> MTIHEHDRVSADRGGDSPHTTHALVDRLMAGEPYAVAFGGQGSAWLETLEELVSATGIETELATLVGEAELLLDPVTDELIVVRPIGFEPLQWVRALAAEDPVPSDKHLTSAAVSVPGVLLTQIAATRALARQGMDLVATPPVAMAGHSQGVLAVEALKAGGARDVELFALAQLIGAAGTLVARRRGISVLGDRPPMVSVTNADPERIGRLLDEFAQDVRTVLPPVLSIRNGRRAVVITGTPEQLSRFELYCRQISEKEEADRKNKVRGGDVFSPVFEPVQVEVGFHTPRLSDGIDIVAGWAEKAGLDVALARELADAILIRKVDWVDEITRVHAAGARWILDLGPGDILTRLTAPVIRGLGIGIVPAATRGGQRNLFTVGATPEVARAWSSYAPTVVRLPDGRVKLSTKFTRLTGRSPILLAGMTPTTVDAKIVAAAANAGHWAELAGGGQVTEEIFGNRIEQMAGLLEPGRTYQFNALFLDPYLWKLQVGGKRLVQKARQSGAAIDGVVISAGIPDLDEAVELIDELGDIGISHVVFKPGTIEQIRSVIRIATEVPTKPVIMHVEGGRAGGHHSWEDLDDLLLATYSELRSRANITVCVGGGIGTPRRAAEYLSGRWAQAYGFPLMPIDGILVGTAAMATKESTTSPSVKRMLVDTQGTDQWISAGKAQGGMASSRSQLGADIHEIDNSASRCGRLLDEVAGDAEAVAERRDEIIAAMAKTAKPYFGDVADMTYLQWLRRYVELAIGEGNSTADTASVGSPWLADTWRDRFEQMLQRAEARLHPQDFGPIQTLFTDAGLLDNPQQAIAALLARYPDAETVQLHPADVPFFVTLCKTLGKPVNFVPVIDQDVRRWWRSDSLWQAHDARYDADAVCIIPGTASVAGITRMDEPVGELLDRF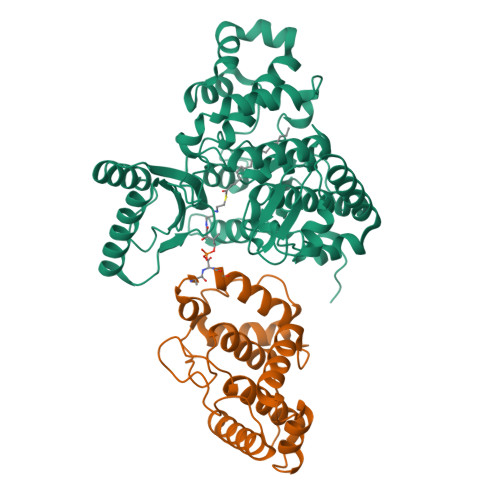EQAAIDEVLGAGVEPKDVASRRLGRADVAGPLAVVLDAPDVRWAGRTVTNPVHRIADPAEWQVHDGPENPRATHSSTGARLQTHGDDVALSVPVSGTWVDIRFTLPANTVDGGTPVIATEDATSAMRTVLAIAAGVDSPEFLPAVANGTATLTVDWHPERVADHTGVTATFGEPLAPSLTNVPDALVGPCWPAVFAAIGSAVTDTGEPVVEGLLSLVHLDHAARVVGQLPTVPAQLTVTATAANATDTDMGRVVPVSVVVTGADGAVIATLEERFAILGRTGSAELADPARAGGAVSANATDTPRRRRRDVTITAPVDMRPFAVVSGDHNPIHTDRAAALLAGLESPIVHGMWLSAAAQHAVTATDGQARPPARLVGWTARFLGMVRPGDEVDFRVERVGIDQGAEIVDVAARVGSDLVMSASARLAAPKTVYAFPGQGIQHKGMGMEVRARSKAARKVWDTADKFTRDTLGFSVLHVVRDNPTSIIASGVHYHHPDGVLYLTQFTQVAMATVAAAQVAEMREQGAFVEGAIACGHSVGEYTALACVTGIYQLEALLEMVFHRGSKMHDIVPRDELGRSNYRLAAIRPSQIDLDDADVPAFVAGIAESTGEFLEIVNFNLRGSQYAIAGTVRGLEALEAEVERRRELTGGRRSFILVPGIDVPFHSRVLRVGVAEFRRSLDRVMPRDADPDLIIGRYIPNLVPRLFTLDRDFIQEIRDLVPAEPLDEILADYDTWLRERPREMARTVFIELLAWQFASPVRWIETQDLLFIEEAAGGLGVERFVEIGVKSSPTVAGLATNTLKLPEYAHSTVEVLNAERDAAVLFATDTDPEPEPEEDEPVAESPAPDVVSEAAPVAPAASSAGPRPDDLVFDAADATLALIALSAKMRIDQIEELDSIESITDGASSRRNQLLVDLGSELNLGAIDGAAESDLAGLRSQVTKLARTYKPYGPVLSDAINDQLRTVLGPSGKRPGAIAERVKKTWELGEGWAKHVTVEVALGTREGSSVRGGAMGHLHEGALADAASVDKVIDAAVASVAARQGVSVALPSAGSGGGATIDAAALSEFTDQITGREGVLASAARLVLGQLGLDDPVNALPAAPDSELIDLVTAELGADWPRLVAPVFDPKKAVVFDDRWASAREDLVKLWLTDEGDIDADWPRLAERFEGAGHVVATQATWWQGKSLAAGRQIHASLYGRIAAGAENPEPGRYGGEVAVVTGASKGSIAASVVARLLDGGATVIATTSKLDEERLAFYRTLYRDHARYGAALWLVAANMASYSDVDALVEWIGTEQTESLGPQSIHIKDAQTPTLLFPFAAPRVVGDLSEAGSRAEMEMKVLLWAVQRLIGGLSTIGAERDIASRLHVVLPGSPNRGMFGGDGAYGEAKSALDAVVSRWHAESSWAARVSLAHALIGWTRGTGLMGHNDAIVAAVEEAGVTTYSTDEMAALLLDLCDAESKVAAARSPIKADLTGGLAEANLDMAELAAKAREQMSAAAAVDEDAEAPGAIAALPSPPRGFTPAPPPQWDDLDVDPADLVVIVGGAEIGPYGSSRTRFEMEVENELSAAGVLELAWTTGLIRWEDDPQPGWYDTESGEMVDESELVQRYHDAVVQRVGIREFVDDGAIDPDHASPLLVSVFLEKDFAFVVSSEADARAFVEFDPEHTVIRPVPDSTDWQVIRKAGTEIRVPRKTKLSRVVGGQIPTGFDPTVWGISADMAGSIDRLAVWNMVATVDAFLSSGFSPAEVMRYVHPSLVANTQGTGMGGGTSMQTMYHGNLLGRNKPNDIFQEVLPNIIAAHVVQSYVGSYGAMIHPVAACATAAVSVEEGVDKIRLGKAQLVVAGGLDDLTLEGIIGFGDMAATADTSMMCGRGIHDSKFSRPNDRRRLGFVEAQGGGTILLARGDLALRMGLPVLAVVAFAQSFGDGVHTSIPAPGLGALGAGRGGKDSPLARALAKLGVAADDVAVISKHDTSTLANDPNETELHERLADALGRSEGAPLFVVSQKSLTGHAKGGAAVFQMMGLCQILRDGVIPPNRSLDCVDDELAGSAHFVWVRDTLRLGGKFPLKAGMLTSLGFGHVSGLVALVHPQAFIASLDPAQRADYQRRADARLLAGQRRLASAIAGGAPMYQRPGDRRFDHHAPERPQEASMLLNPAARLGDGEAYIG;> MTIHEHDRVSADRGGDSPHTTHALVDRLMAGEPYAVAFGGQGSAWLETLEELVSATGIETELATLVGEAELLLDPVTDELIVVRPIGFEPLQWVRALAAEDPVPSDKHLTSAAVSVPGVLLTQIAATRALARQGMDLVATPPVAMAGHSQGVLAVEALKAGGARDVELFALAQLIGAAGTLVARRRGISVLGDRPPMVSVTNADPERIGRLLDEFAQDVRTVLPPVLSIRNGRRAVVITGTPEQLSRFELYCRQISEKEEADRKNKVRGGDVFSPVFEPVQVEVGFHTPRLSDGIDIVAGWAEKAGLDVALARELADAILIRKVDWVDEITRVHAAGARWILDLGPGDILTRLTAPVIRGLGIGIVPAATRGGQRNLFTVGATPEVARAWSSYAPTVVRLPDGRVKLSTKFTRLTGRSPILLAGMTPTTVDAKIVAAAANAGHWAELAGGGQVTEEIFGNRIEQMAGLLEPGRTYQFNALFLDPYLWKLQVGGKRLVQKARQSGAAIDGVVISAGIPDLDEAVELIDELGDIGISHVVFKPGTIEQIRSVIRIATEVPTKPVIMHVEGGRAGGHHSWEDLDDLLLATYSELRSRANITVCVGGGIGTPRRAAEYLSGRWAQAYGFPLMPIDGILVGTAAMATKESTTSPSVKRMLVDTQGTDQWISAGKAQGGMASSRSQLGADIHEIDNSASRCGRLLDEVAGDAEAVAERRDEIIAAMAKTAKPYFGDVADMTYLQWLRRYVELAIGEGNSTADTASVGSPWLADTWRDRFEQMLQRAEARLHPQDFGPIQTLFTDAGLLDNPQQAIAALLARYPDAETVQLHPADVPFFVTLCKTLGKPVNFVPVIDQDVRRWWRSDSLWQAHDARYDADAVCIIPGTASVAGITRMDEPVGELLDRFEQAAIDEVLGAGVEPKDVASRRLGRADVAGPLAVVLDAPDVRWAGRTVTNPVHRIADPAEWQVHDGPENPRATHSSTGARLQTHGDDVALSVPVSGTWVDIRFTLPANTVDGGTPVIATEDATSAMRTVLAIAAGVDSPEFLPAVANGTATLTVDWHPERVADHTGVTATFGEPLAPSLTNVPDALVGPCWPAVFAAIGSAVTDTGEPVVEGLLSLVHLDHAARVVGQLPTVPAQLTVTATAANATDTDMGRVVPVSVVVTGADGAVIATLEERFAILGRTGSAELADPARAGGAVSANATDTPRRRRRDVTITAPVDMRPFAVVSGDHNPIHTDRAAALLAGLESPIVHGMWLSAAAQHAVTATDGQARPPARLVGWTARFLGMVRPGDEVDFRVERVGIDQGAEIVDVAARVGSDLVMSASARLAAPKTVYAFPGQGIQHKGMGMEVRARSKAARKVWDTADKFTRDTLGFSVLHVVRDNPTSIIASGVHYHHPDGVLYLTQFTQVAMATVAAAQVAEMREQGAFVEGAIACGHSVGEYTALACVTGIYQLEALLEMVFHRGSKMHDIVPRDELGRSNYRLAAIRPSQIDLDDADVPAFVAGIAESTGEFLEIVNFNLRGSQYAIAGTVRGLEALEAEVERRRELTGGRRSFILVPGIDVPFHSRVLRVGVAEFRRSLDRVMPRDADPDLIIGRYIPNLVPRLFTLDRDFIQEIRDLVPAEPLDEILADYDTWLRERPREMARTVFIELLAWQFASPVRWIETQDLLFIEEAAGGLGVERFVEIGVKSSPTVAGLATNTLKLPEYAHSTVEVLNAERDAAVLFATDTDPEPEPEEDEPVAESPAPDVVSEAAPVAPAASSAGPRPDDLVFDAADATLALIALSAKMRIDQIEELDSIESITDGAXSRRNQLLVDLGSELNLGAIDGAAESDLAGLRSQVTKLARTYKPYGPVLSDAINDQLRTVLGPSGKRPGAIAERVKKTWELGEGWAKHVTVEVALGTREGSSVRGGAMGHLHEGALADAASVDKVIDAAVASVAARQGVSVALPSAGSGGGATIDAAALSEFTDQITGREGVLASAARLVLGQLGLDDPVNALPAAPDSELIDLVTAELGADWPRLVAPVFDPKKAVVFDDRWASAREDLVKLWLTDEGDIDADWPRLAERFEGAGHVVATQATWWQGKSLAAGRQIHASLYGRIAAGAENPEPGRYGGEVAVVTGASKGSIAASVVARLLDGGATVIATTSKLDEERLAFYRTLYRDHARYGAALWLVAANMASYSDVDALVEWIGTEQTESLGPQSIHIKDAQTPTLLFPFAAPRVVGDLSEAGSRAEMEMKVLLWAVQRLIGGLSTIGAERDIASRLHVVLPGSPNRGMFGGDGAYGEAKSALDAVVSRWHAESSWAARVSLAHALIGWTRGTGLMGHNDAIVAAVEEAGVTTYSTDEMAALLLDLCDAESKVAAARSPIKADLTGGLAEANLDMAELAAKAREQMSAAAAVDEDAEAPGAIAALPSPPRGFTPAPPPQWDDLDVDPADLVVIVGGAEIGPYGSSRTRFEMEVENELSAAGVLELAWTTGLIRWEDDPQPGWYDTESGEMVDESELVQRYHDAVVQRVGIREFVDDGAIDPDHASPLLVSVFLEKDFAFVVSSEADARAFVEFDPEHTVIRPVPDSTDWQVIRKAGTEIRVPRKTKLSRVVGGQIPTGFDPTVWGISADMAGSIDRLAVWNMVATVDAFLSSGFSPAEVMRYVHPSLVANTQGTGMGGGTSMQTMYHGNLLGRNKPNDIFQEVLPNIIAAHVVQSYVGSYGAMIHPVAACATAAVSVEEGVDKIRLGKAQLVVAGGLDDLTLEGIIGFGDMAATADTSMMCGRGIHDSKFSRPNDRRRLGFVEAQGGGTILLARGDLALRMGLPVLAVVAFAQSFGDGVHTSIPAPGLGALGAGRGGKDSPLARALAKLGVAADDVAVISKHDTSTLANDPNETELHERLADALGRSEGAPLFVVSQKSLTGHAKGGAAVFQMMGLCQILRDGVIPPNRSLDCVDDELAGSAHFVWVRDTLRLGGKFPLKAGMLTSLGFGHVSGLVALVHPQAFIASLDPAQRADYQRRADARLLAGQRRLASAIAGGAPMYQRPGDRRFDHHAPERPQEASMLLNPAARLGDGEAYIG One of these is a hybrid heme peroxidase, the T. cruzi ascorbate peroxidase-cytochrome c peroxidase enzyme (TcAPx-CcP). TcAPx-CcP has high sequence identity to members of the class I peroxidase family, notably ascorbate peroxidase (APX) and cytochrome c peroxidase (CcP), as well as a mitochondrial peroxidase from Leishmania major (LmP). Like LmP, TcAPx was later found to have both ascorbate and cytochrome c activity and was thus renamed as TcAPx-CcP. Integration of steady state kinetic experiments, molecular dynamic simulations, and bioinformatic analyses indicates that TcAPx-CcP preferentially oxidizes cytochrome c but is still competent for oxidization of ascorbate.

On the proximal side there is a typical peroxidase His217-Asp278-Trp233 proximal triad, as observed in yeast CcP and in soybean APX (sAPX, His163-Asp208-Trp179). Electron paramagnetic resonance (EPR) was used to assess whether TcAPx-CcP uses the corresponding Trp233 radical. EPR spectra taken at 4 K for TcAPx-CcP on reaction with H2O2 are consistent with the formation of a [Fe(IV)=O Trp•+] radical in compound I, with a concomitant reduction of the high spin iron heme, g = 6, signal (Fig. 3Ai-ii). The radical was centered at g = 2 and showed a pronounced broad linewidth only present at the lowest temperatures with a narrower radical signal observed at 70 K (Fig. 3B(i)). Similar EPR spectra were reported for the exchange coupled porphyrin-tryptophanyl radical in LmP. This broadening was clearly absent in parallel experiments at 4 K on the W233F variant (Fig. 3Aiii-iv). There are two molecules in the asymmetric unit for both the wild type and mutant structures, each one exhibiting different electron density at the distal heme position, with one appearing to bind an oxygen molecule and another a water molecule approximately 2.3 Å above the iron (not shown). The low temperature EPR spectra support the formation of a reactive compound I intermediate with an exchange-coupled [Fe(IV)=O Trp233•+] radical.

>[2x]MAFCFGSFFSKYASSKSGSQARYRFLHSSAKIAAGATGALLLGGATVALCYFPSGRKVTEAPPFDVNSLRRDIEEILSEDMSKGPLFVRLAWHEAGSWDCRKKDGSPNSASMRFHPECSYAGNKGLDKGRNALESLKKKYPKISYADLWSFAAVVSIEAMGGPEIPWRWGRVDAKDGSVCGPDGRLPDASRMQDHVRDVFSRLGFNDEETVALIGAHTCGECHLENTGYVGPFTHDKYGFDNSFFTELFGNEWMLNPNVKKMQFMDKTTNRLMMLPADVSILLDDKYRSIAKKYADDNDYFCNAFSKAYQKLLEVGTTDLKSLPAESK5-METHYL-7-(2-METHYLPROPYL)-2-(NAPHTHALEN-1-YLMETHYL)-3-PYRIDIN-4-YL-2H-PYRAZOLO[3,4-D]PYRIMIDINE-4,6(5H,7H)-DIONE 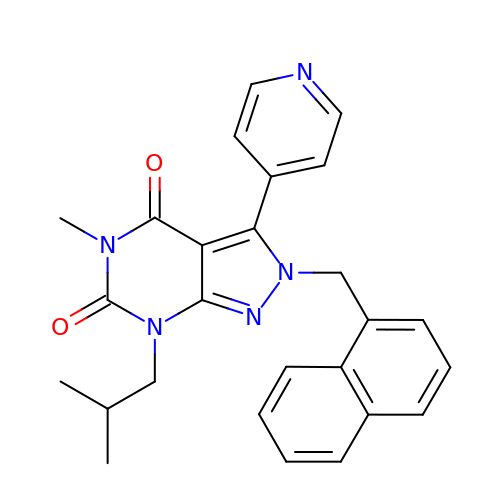| C26 H25 N5 O2 | NNZDBCPMOOEFTE-UHFFFAOYSA-N4-tert-butyl-N-(2-methyl-3-{2-[4-(morpholine-4-carbonyl)phenyl]-1H-imidazo[4,5-b]pyridin-7-yl}phenyl)benzamide | C35 H35 N5 O3 | 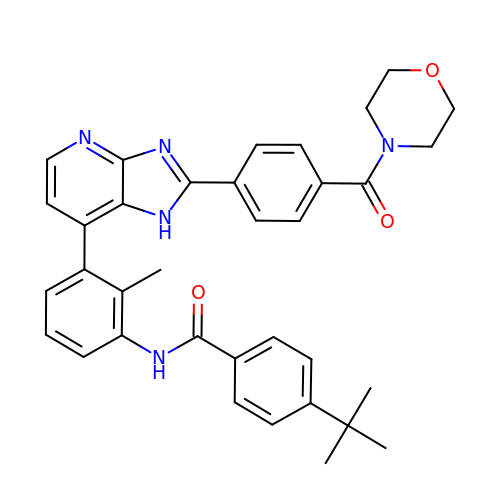CMNOPGSZOYYDCD-UHFFFAOYSA-N>[2x]MNNRVHQGHLARKRFGQNFLNDQFVIDSIVSAINPQKGQAMVEIGPGLAALTEPVGERLDQLTVIELDRDLAARLQTHPFLGPKLTIYQQDAMTFNFGELAEKMGQPLRVFGNPPYNISTPLMFHLFSYTDAIADMHFMLQKEVVNRLVAGPNSKAYGRLSVMAQYYCNVIPVLEVPPSAFTPPPKVDSAVVRLVPHATMPHPVKDVRVLSRITTEAFNQRRKTIRNSLGNLFSVEVLTGMGI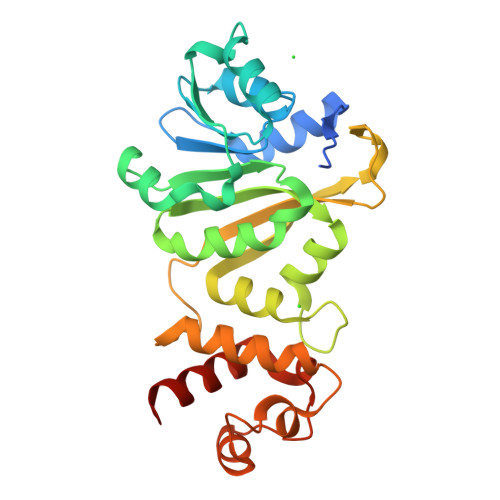DPAMRAENISVAQYCQMANYLAENAPLQES> MLGILNKMFDPTKRTLNRYEKIANDIDAIRGDYENLSDDALKHKTIEFKERLEKGATTDDLLVEAFAVVREASRRVTGMFPFKVQLMGGVALHDGNIAEMKTGEGKTLTSTLPVYLNALTGKGVHVVTVNEYLASRDAEQMGKIFEFLGLTVGLNLNSMSKDEKREAYAADITYSTNNELGFDYLRDNMVLYKEQMVQRPLHFAVIDEVDSILIDEARTPLIISGQAAKSTKLYVQANAFVRTLKAEKDYTYDIKTKAVQLTEEGMTKAEKAFGIDNLFDVKHVALNHHINQALKAHVAMQKDVDYVVEDGQVVIVDSFTGRLMKGRRYSEGLHQAIEAKEGLEIQNESMTLATITFQNYFRMYEKLAGMTGTAKTEEEEFRNIYNMQVVTIPTNRPVVRDDRPDLIYRTMEGKFKAVAEDVAQRYMTGQPVLVGTVAVETSELISKLLKNKGIPHQVLNAKNHEREAQIIEEAGQKGAVTIATNMAGRGTDIKLGEGVKELGGLAVVGTERHESRRIDNQLRGRSGRQGDPGITQFYLSMEDELMRRFGAERTMAMLDRFGMDDSTPIQSKMVSRAVESSQKRVEGNNFDSRKQLLQYDDVLRQQREVIYKQRFEVIDSENLREIVENMIKSSLERAIAAYTPREELPEEWKLDGLVDLINTTYLDEGALEKSDIFGKEPDEMLELIMDRIITKYNEKEEQFGKEQMREFEKVIVLRAVDSKWMDHIDAMDQL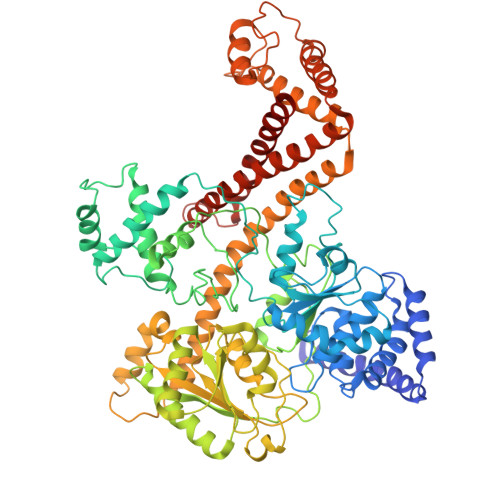RQGIHLRAYAQTNPLREYQMEGFAMFEHMIESIEDEVAKFVMKAE>SNAAAAAFESVIEEHDIPGLVVGVTHGGRHSFYQTGLASREDQQPVTPDTLFELGSISKIFNVTLAALAEERGALSLDAPVADYLPSLRGSPAGELTLIDLATHHTGGLPLQVPDEVADVDRLVDWLRSWRPPEPGTRSYSNISIGLLGHITAGVLGMSYADASQTVIFPALGLKSTWIDVPTDAMGRYAFGYDRKTDAPTRVTPGVLDDEAYGVKSSARDMLTL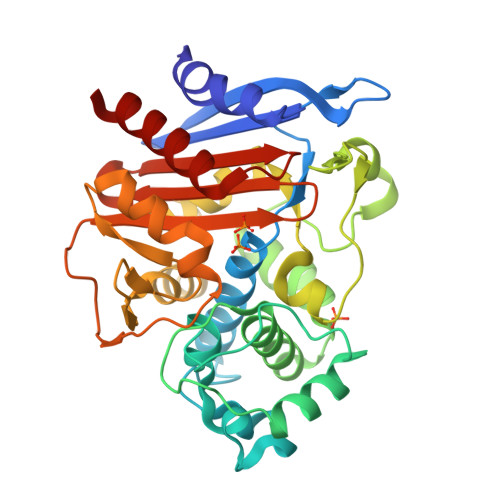LDLELGTGTASPEVQTAVATTQEGRFQTRLYTQAMIWEAYPWPVDPERLVEGNGYDFILQPQPVDEVDTTPDRRVILNKTGSTNGFGGYIAIVPSEDLGVVVLANRNYPNEARVRATYDLITHILA[2x]Previous studies showed that repetitive interspersed family (RIFIN) proteins, displayed on the surfaces of Plasmodium falciparum-infected erythrocytes, can bind to inhibitory immune receptors and dampen NK cell activation, reducing parasite killing. Killer immunoglobulin-like receptors (KIRs) are expressed on NK cells and consist of pairs of inhibitory and activating immune receptors. Here we identified a clade of RIFINs that bind to inhibitory immune receptor KIR2DL1 more strongly than KIR2DL1 binds to the human ligand (MHC class I). To show how RIFINs bind to KIR2DL1, we determined the structures of RBK21 and KEN-01, each bound to KIR2DL1.

For RBK21, the variable region (residues 148–299) was mixed with the KIR2DL1 ectodomain and crystallized. The variable regions of both RBK21 and KEN-01 consisted of a helical bundle that presented extended loops and short helices at the KIR-proximal end. In both cases, the KIR2DL1 binding site was formed from two helices and two loops, which contacted the D1 domain of KIR2DL1, with a conserved binding pose despite only 53% of the KIR2DL1-contacting residues being shared. The binding site was centred around a conserved hydrophobic core, with L224 and F242 from each RIFIN occupying a shallow hydrophobic pocket containing residues L59, Y101 and V111 of KIR2DL1. This was stabilized by an intermolecular β-sheet, which contained loop 4 of RBK21 or KEN-01 and ended with a hydrogen bond linking S258 of RBK21 or KEN-01 and D68 of KIR2DL1. In RBK21, residue S221 was at the centre of the interface. To develop a non-binding mutant of RBK21 for future studies, we produced S221R. This abolished binding to KIR2DL1, as shown by SPR analysis, despite circular dichroism indicating that it adopted the correct fold. Inspection of the RBK21–KIR2DL1 structure showed that the KIR2DL1 residues, which interact with RBK21, were almost completely conserved in KIR2DS1, except for the conservative substitution of V111L.

>[8x]VALAKAIAEGAAKGAEVGEAARIAAAIDAVIKGIETKFGVSTNGVLGLKSLFTANNYNNATKIAGAIIEEYKPSSCLTGGSGADNSICPWAMENFFAARKIPGFIQREAVSMNDVIEKTVKTIVSDAPKTAETAAKKATEEAIKASTDAVES;>[8x]RKPSLLAHPGPLVKSEETVILQCWSDVMFEHFLLHREGMFNDTLRLIGEHHDGVSKANFSISRMTQDLAGTYRCYGSVTHSPYQVSAPSDPLDIVIIGLYEKPSLSAQPGPTVLAGENVTLSCSSRSSYDMYHLSREGEAHERRLPAGPKVNGTFQADFPLGPATHGGTYRCFGSFHDSPYEWSKSSDPLLVSVT> MTQTQTAARTFVDTVTYRPGAVILYPGKSDMLYRVSSGLVRVHTMDDDGNGLTLRYVKPGEYFGEEALAGVNRAYFAEAVTDSAIDVINPALMSAEDNLVVTTHLVRTLERAYESIYRLVGKRLRARIAGELLELKDTALATQLDSGETMIYATHDELAAAVGSVRETVTKVVGELSREGVISAGYGKITLKDERALATIAAA

The cAMP receptor proteins (CRPs) play a critical role in bacterial environmental adaptation by regulating global gene expression levels via cAMP binding. Here, we report the structure of DdrI, a CRP family protein from Deinococcus radiodurans. Combined with biochemical, kinetic, and molecular dynamics simulations analyses, our results indicate that DdrI adopts a DNA-binding conformation in the absence of cAMP and can form stable complexes with the target DNA sequence of classical CRPs. Among these candidates, DdrI was identified as playing a major role in global regulation for the adaptation of D. radiodurans to various stresses. ddrI was highly induced by gamma radiation treatments, and the inactivation of this gene sensitized cells to various stress environments including heat shock, radiation, DNA-damaging agents, and oxidation.

DdrI crystals were grown and diffracted X-rays to 2.0 Å. While the asymmetric unit contains one DdrI monomer, two neighboring molecules form a dimer, consistent with its dimerization in solution. The final model, which comprises 7 α-helices and 12 β-strands, contains two domains: a nucleotide-binding N-terminal domain (NDB, residues 13–94) and a DNA-binding C-terminal domain (DBD, residues 122–202). These two domains are interconnected by a long linker α-helix (C-helix; residues 95–121). The NDB of DdrI shares a canonical jelly roll topology with two layers of antiparallel β-strands, and DBD contains a winged HTH motif (E- and F-helices) critical for DNA binding. Importantly, the linker C-helix in the DdrI structure is fully folded, in contrast to the partial folding of this region in ecCRP in the absence of cAMP. Thus, the fully folded C-helix of apo DdrI led us to suspect that our DdrI without cAMP binding represents the active CRP form. Notably, compared with ecCRP apo structure lacking the cAMP, the β4-β5 loop and D-helix show noticeable movement, with the F-helix being in a position compatible with target DNA binding. In contrast to the cavity occupied by the cAMP molecule in ecCRP, this binding pocket of DdrI is partially filled with Tyr113n-Arg55-Glu65 (equivalent to ecCRP Ser128n, Ser62, and Glu72). Instead of interacting with the adenine base as its ecCRP equivalent does, Arg55 of DdrI forms hydrogen bonds with both Tyr113n and Glu65, leading to insufficient space for cAMP accommodation.>ADPGAAPSYQALPAGNLCPAAAYDSRYNTKYLGFFTHLVQAQDDWLFRTTYDLRTDFGTSAEGWRELRALRDELKRKGIELVVVYQPTRGLVNREKLSPAEKAGFDYELAKKNYLATIARFRQAGIWTPDFSPLFDEKEEHAYYFKGDHHWTPHGARRSAKIVAETLKQVPGFEEIPKKQFESKRVGLLSKLGTFHKAAAQLCGNSYATQYVDRFETEPVGASDSGDLFGDGGNPQIALVGTSNSGPAYNFAGFLEEFSGADILNNAVSGGGFDSSLLAYMTSEEFHKNPPKILIWEFATHYDMAQKSFYRQAMPLVDNGCSGRKTVLSRKVKLRQGRNEVLLNSAALPIRSGS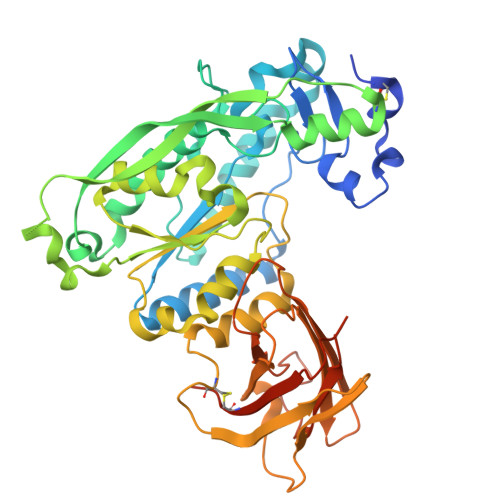YVADVTYSDPSVHELKNTIWYMNGRREQLKIEQSKAVDTGGRYVFQLRNDSDWADQQFLSLEIEAPEDMPQGLEVQASICQAAPAKASQSVAGRLEHHHHHH[2x]5-fluoro-2-{4-[(methylamino)methyl]phenyl}-1-benzofuran-7-carboxamide | C17 H15 F 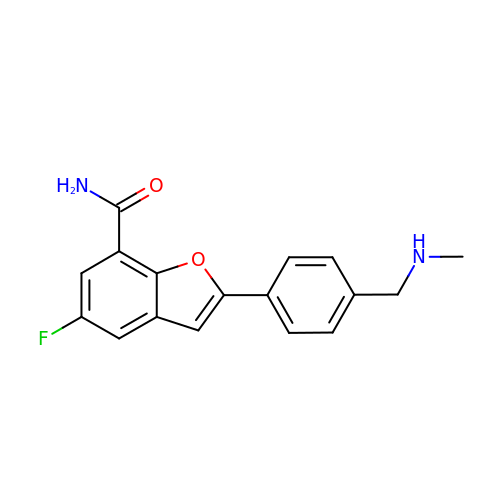N2 O2 | ROBJKLPZIPNAMV-UHFFFAOYSA-N> GSHMGLFNAHAVAQQRADRIATLLQSFADGQLDTAVGEAPAPGYERLYDSLR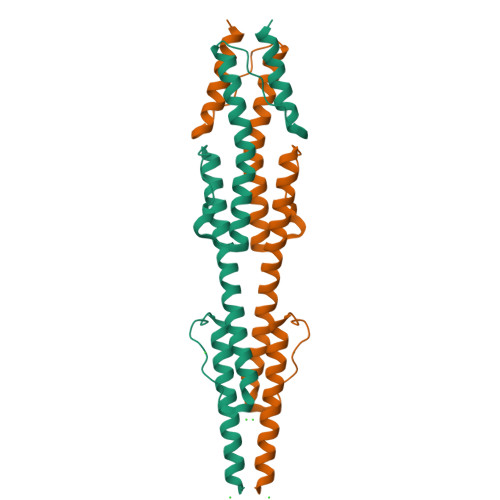ALQRQLREQRAELQQVESLEAGLAEMSRQHEAGWIDQTIPAERLEGRAARIAKGVNELVAAHIAVKMKVVSVVTAYGQGNFEPLMDRLPGKKAQITEAIDGVRERLRGAAEATSAQLATAAYN5'-S-[3-(N'-benzylcarbamimidamido)propyl]-5'-thioadenosine | C21 H28 N8 O3 S | 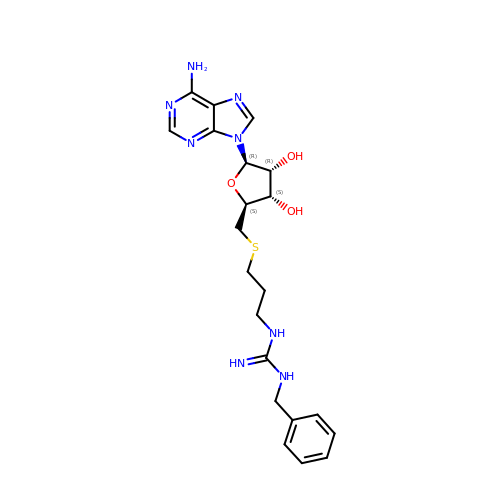LTPOXWXTHQVJKG-WVSUBDOOSA-N> HHHHHHGSGLKVRLVGGSGPHEGRVEILHSGQWGTICDDRWEVRVGQVVCRSLGYPGVQAVHKAAHFGQG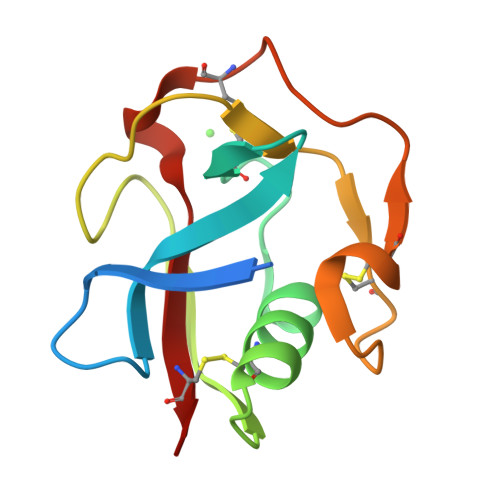TGPIWLNEVFCFGRESSIEECKIRQWGTRACSHSEDAGVTCTL> MSWQAYVDDHLMCEIEGNHLSAAAIIGQDGSVWAQSANFPQFKSEEITGIMSDFHEPGTLAPTGLYIGGTKYMVIQGEPGAVIRGKKGPGGVTVKKTNQALI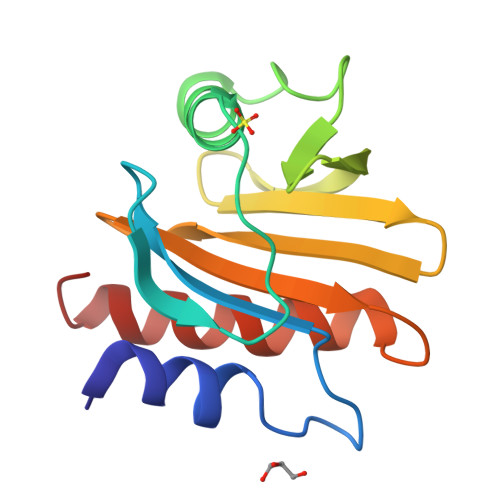IGIYDEPMTPGQCNMIVERLGDYLIDQGY> PGEWAGKDKIEKVSIYM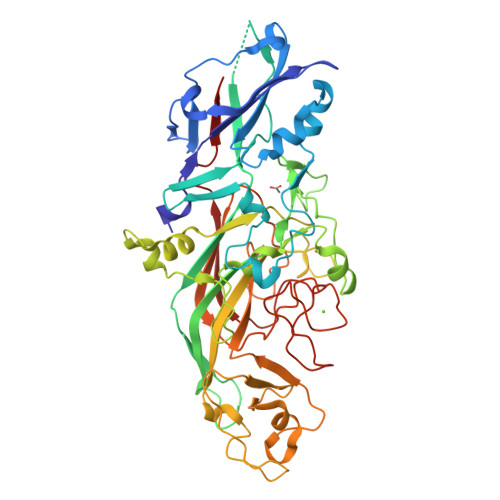VPQGGPGLVESAEDLDFGTYYENPTIDPATHNAILKPKKGIKVNSAVGKTVKVYVVLNDIAGKAKALLANVNAADFDAKFKEIIELSTQAQALGTVADGPNPATAAGKIAKKNGTTDETIMMTCLQPSDALTIEEAAVSEANAIAGIKNQAKVTVERSVARAMVSTKAQSYEIKATTQIGEIAAGSVLATITDIRWVVAQGERRQYLSKKRGTVPENTWVTPGSGFVPTSSTFHTNATEYYDYAGLWEDHNTNEAVISGTQVPTLADYQLQDVTGELANALSGKFLLPNTHKSGANAASSDYKRGNTAYVLVRAKFTPKKEAFIDRGKTYSDNTAVPEYVAGEDFFVGENGQFYVSMKSVTDPKVGGVAGMKAHKYVKGKVLYYAWLNPSTTSPDSWWNSPVVRNNIYHIHIKSIKKLGFNWNPLVPDPDPSNPENPNNPDPNPDEPGTPVPTDPENPLPDQDTFMSVEVTVLPWKVHSYEVDL>GEEPVPVPTEQTVFMYLPWSDNLTSNFYQNISDLESVVEKNILKDERIIIFMCTTATKATLFELAYENGKSVHKTLKNYTDPAYTTAEGITSILNDVQRYSPTKRYSMVIGCHGMGWIPVSNSKSASGLRTKMHWE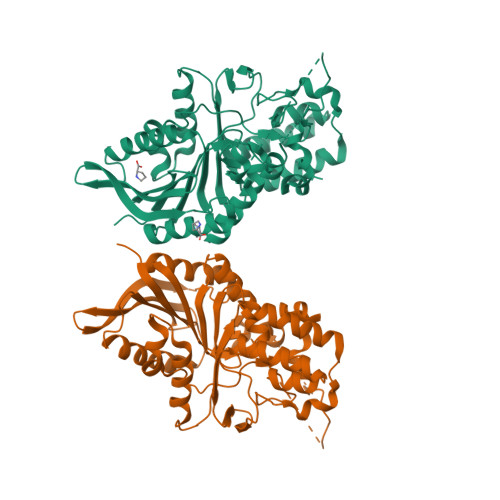YENVPMTRYFGGLNAQYQTDITTLAKGISNAGLKMEYILFDDCYMSSIEVAYALKDVTDYLIGSTSEVMAYGMPYAEIGQYLIGKVDYAGICDGFYSFYSTYSTPCGTIAVTDCSELDNLATIMKEINHRYTFDPSLTSSLQRLDGYYPVIFFDYGDYVSKLCPDETLVARFNEQLNRTVPFKRNTEYFYSMSRGEVKINTFSGITISDPSTHSLASKKEETAWYAATH[2x]> MAPKGTSLDEKKERLLEEMLKRGEIYSNKTIETLSKPTGISSMVIKNVLQALVNEDLVDTDKIGASTYYWCFASKRSQ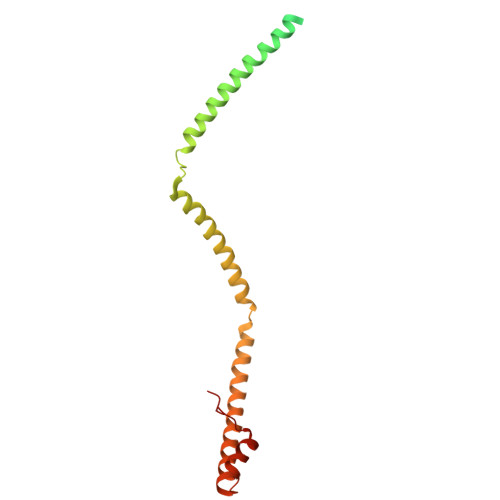AARTELARLQKALEEQTNFIDKATARIEELKVGREETEERSSLLKEKLALQVKLEEQRGTFRDLLKNDPDVAQKLRNYTDIAKQEANLWTDNIFCLQKYMLTKLQMDKKTVSTALGITGEFDYLE>[3x]GGVTDALSLMYSTSTGGPASIA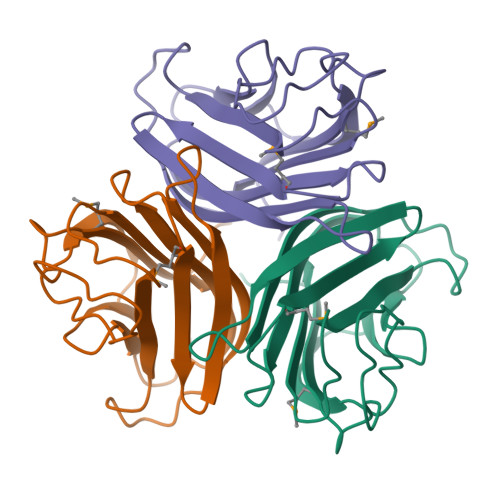ANALTDFDLSGALTVNSVGTGLTKSAAGIQLAAGKSGLYQITMTVKNNTVTTGNYLLRVKYGSSDFVVACPASSLTAGGTISLLIYCNVLGVVSLDVLKFSLCNDGAALSNYIINITAAKIN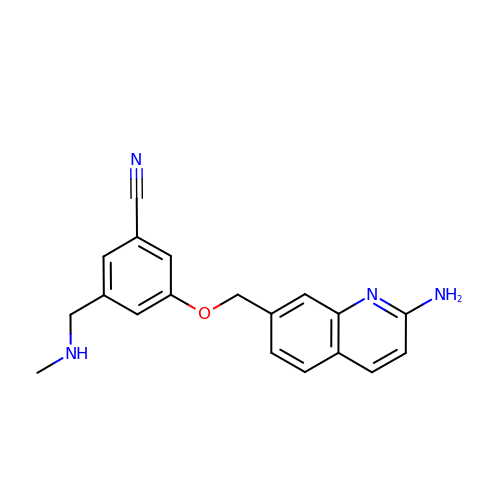3-[(2-aminoquinolin-7-yl)methoxy]-5-[(methylamino)methyl]benzonitrile | C19 H18 N4 O | QYHMAWINXHLCMX-UHFFFAOYSA-N> MLGGLRPLAAATRRTVGGALVSPALITPSRALSVRTEDFFSKEAVSHARRVSWAPHTTEKKVGAFAKLSRSNFNDPLPVSFQSEPYFEEEIEAYRA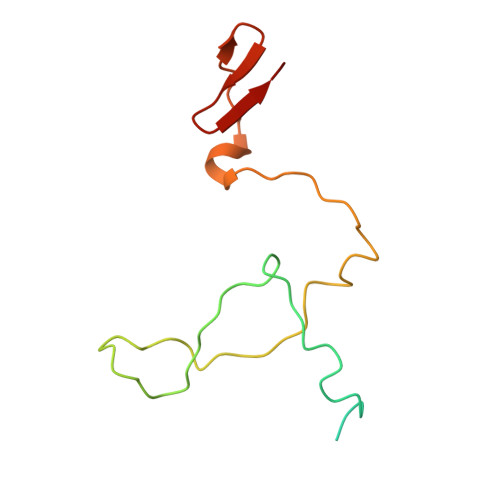HHRPDVYVYKYNVSPTHLSLRE By targeting its receptors C5aR1 and C5aR2 on a wide range of immune cells69 as well as endothelial cells10, C5a promotes inflammation, vascular permeability and coagulation. Mirror-image aptamers, also referred to as Spiegelmers (from German Spiegel=mirror), possess the high target specificity of conventional aptamers and are in addition plasma nuclease resistant, therefore having high therapeutic and diagnostic potential. Here we report the crystal structures of NOX-D20 in complex with either murine C5a (mC5a) or its C-terminally desarginylated version mC5a-desArg, at 1.8 and 2.0 Å resolution, respectively. The structures reveal a complex 3D architecture for the Spiegelmer, including a left-turning double-helix and an intramolecular G-quadruplex stabilized by a Ca2+ ion.

The structure of the NOX-D20:mC5a complex was determined by single-wavelength anomalous diffraction (SAD) phasing using crystals derivatized with Os(NH3)6. Unexpectedly, the asymmetric units of both NOX-D20:mC5a and NOX-D20:mC5a-desArg crystals contained three molecules of mC5a and only two molecules of NOX-D20. The final models encompass residues Asn679 to Pro750 for mC5a, Asn679 to Lys744 for mC5a-desArg and all 40 nucleotides for the Spiegelmer. NOX-D20 folds into a compact V-shape with the concave face of the V wrapping around the C5a molecule along the H1-H2-H3 side. The two binding partners display a strong shape complementarity, resulting in a total surface area buried at the NOX-D20:mC5a interface of 1,791 Å2, as estimated with AREAIMOL24. The two Ca2+ surrounding the Mg2+ ion are heptacoordinated by water molecules, oxygens from the phosphate groups of U5, G6, C31 and C34 and, for the most peripheral calcium ion, by the side chain of Asp705 protruding from mC5a helix H2. Within the complex, mC5a inserts into the V-shaped groove formed at the interface between the two structural domains of NOX-D20 and the Spiegelmer's binding pocket almost perfectly complements the surface shape of mC5a helices H1, H2 and H3. Lys701 and Asp705, located in the middle of H2, form hydrogen bonds with U5 and G32 phosphate groups, along the minor groove of the NOX-D20 stem domain, and with the base of dU28. Comparison of the footprint of NOX-D20 onto mC5a with the position of the C5a residues presumably involved in C5aR binding reveals that NOX-D20 strongly overlaps with the first C5aR-binding site.

>GANLHLLRQKIEEQAAKYKHSVPKKCCYDGARVNFYETCEERVARVTIGPLCIRAFNECCTIANKIRKESPHKPVQLGR[3x]7-{[3-({[2-(pyridin-2-yl)ethyl]amino}methyl)phenoxy]methyl}quinolin-2-amine 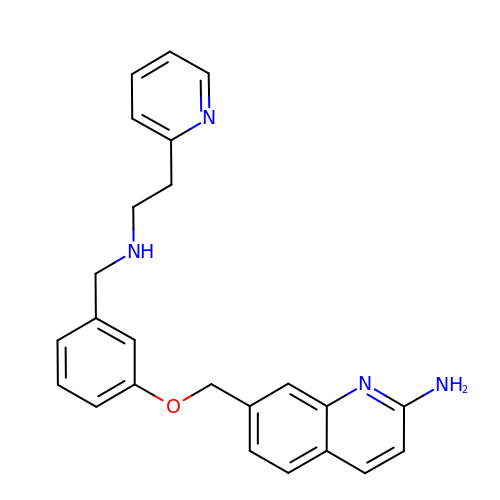| C24 H24 N4 O | VWEIPCRIPQWNJS-UHFFFAOYSA-N> GDIVMKEKPKVTLNEIVGLEDVKEALKEAVVYPSKRPDLFPLGWPRGILLYGPPGCGKTMIAAAVANELDSEFIHVDAASIMSKWLGEAEKNVAKIFKTARELSKKENKPAIIFIDELDALLASYTSEVGGEARVRNQFLKEMDGLADKNEISKVYVIGATNKPWRLDEPFLRRFQKRIYITLPDKAHRLELLKHYSSKVKLDPNVNLEELAELTDGYTASDIRDIVQSAHMRVVKEMFEKNLQEPRAINMDDFREVLKVRKPSVNQDMLKAYAAWHEKFKAL

Vps4, a member of the type-I or meiotic clade of AAA family of proteins (ATPase associated with various activities)11 disassembles ESCRT-III polymers from membranes, which might be coupled to the membrane fission reaction itself. Proteins homologous to Vps4 and ESCRT-III are also present in the Crenarchaeota phylum of archaea where they catalyse final steps in cell division, virus budding and vesicle release. Vps4 contains an amino-terminal microtubule interacting and trafficking (MIT) domain that interacts with carboxy-terminal peptide motifs termed MIT domain-interacting motif in activated eukaryotic and archaeal ESCRT-III proteins. Here we characterized the oligomeric state of the Vps4 homologue from M. sedula (MsVps4) that belongs to the phylum Crenarchaeota.

To probe the conformation on nucleotide binding, hexameric MsVps4ΔMIT and a shorter MsVps4 construct lacking the linker region (MsVps4ΔL-MIT, residues 88–369) were crystallized in the presence of ADP and Mg2+. Both constructs crystallized with P65 helical symmetry with similar H interfaces as observed in the hexamer structure and a V interface close the to A–B interface. ADP is coordinated between the large and small ATPase domains and P-loop residues Gly141, Cys142, Gly143, Lys144 and Thr145 (located on the large ATPase domain) bind the α- and β-phosphate groups of ADP, whereas Tyr282, Arg310 and Val103 (located on the small ATPase domain) make hydrogen bonds with the sugar and the base. The base is stacked between the small and large ATPase domain in a pocket composed of residues Met146, Leu278 and Ala306. Comparison of the nucleotide-free apo structure present in the ring structure showed that ADP binding induced a 23° rotation of the small ATPase domain compared with the large one. ADP bound to MsVps4 occupies a similar position as ATPγS bound to yeast Vps4p, whereas ADP bound to yeast Vps4p penetrates less into the binding pocket. The N-terminal region comprising residues 88–95 is disordered in the ring structure but form a short β′-strand and α-helix in the ADP-bound monomer structure, thus possibly acting as a flexible arm helping to reorient the MIT domain and its bound substrate during the ATP cycle. Our crystal structures reveal that the β′-strand at the N terminus is ordered in the ADP-bound conformation and disordered in the nucleotide-free conformation, suggesting that this conformational flexibility might be important for MIT domain orientation.In order to decipher the structural basis of their substrate specificities and to provide a rational, we structurally and biochemically characterized two 1β aminotransferases from Mycobacterium tuberculosis (Mtb), an HspAT, encoded by rv1600 (mHspAT) and a putative phenylalanine aminotransferase, encoded by rv3772. However, experimental characterisation of this aminotransferase in the current study clearly demonstrates high catalytic preference for Phe, Tyr and Trp instead for Hsp. Therefore, we propose its reannotation of as an aromatic amino acid aminotransferase (mArAT). Contrastingly in mArAT, residues Val86, Phe110, Leu112 and Phe246* form a hydrophobic substrate binding pocket which provides an energetically favourable environment for the specific binding of hydrophobic substrates such as Phe, Trp and the less polar Tyr.

The binding of Phe and succinate in the active site of mArAT as observed in the crystal structures of mArAT-PLP-Phe and mArAT-PMP-succinate complexes revealed the molecular basis of substrate selectivity of mArAT. The two liganded structures are virtually identical (an rmsd of 0.28 Å over 305 Cα atom pairs). As seen in the one of the mArAT crystal structure, a dicarboxylic acid, succinate was bound in the active site pocket. In the dicarboxylate bound form, succinate exists as a non-covalently linked moiety, forming a ‘twisted’ bidentate H-bond/ion pair with Arg322 and Arg330 of the C-terminal domain. Succinate essentially mimics L-glutamate, an amino donor. Utilizing the structural information gained from the two structures, we traced the plausible conformational changes that mArAT undergoes - from accommodating a dicarboxylate to creating a suitable cavity for Phe entry and binding. Thus, the first choice of molecules for inhibition studies were the dicarboxylate molecules succinic acid and maleic acid, the latter being a well-studied inhibitor of aminotransferases. However, both the dicarboxylates failed to inhibit mHspAT and mArAT.

>[4x]MVTARLRPELAGLPVYVPGKTVPGAIKLASNETVFGPLPSVRAAIDRATDTVNRYPDNGCVQLKAALARHLGPDFAPEHVAVGCGSVSLCQQLVQVTASVGDEVVFGWRSFELYPPQVRVAGAIPIQVPLTDHTFDLYAMLATVTDRTRLIFVCNPNNPTSTVVGPDALARFVEAVPAHILIAIDEAYVEYIRDGMRPDSLGLVRAHNNVVVLRTFSKAYGLAGLRIGYAIGHPDVITALDKVYVPFTVSSIGQAAAIASLDAADELLARTDTVVAERARVSAELRAAGFTLPPSQANFVWLPLGSRTQDFVEQAADARIVVRPYGTDGVRVTVAAPEENDAFLRFARRWRSDQKLAAALEHHHHHH>[1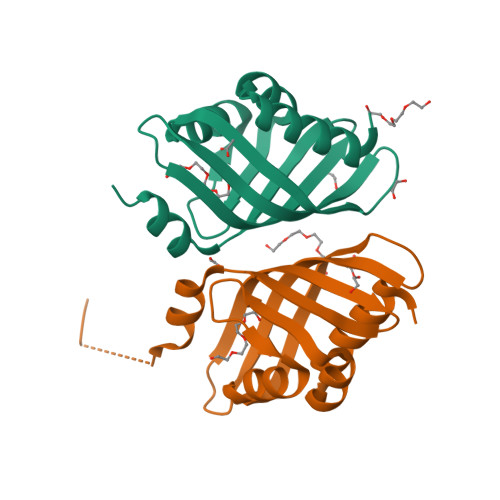6x]MTPLETVQLFLARVNALDLDGACALLAEDVVYDNVPMPTVHGRAAARAFLSQLPATAIDWETHAIAATGDAARGTVLTERTDRFTLADGRTLAIRVMGAFDVADGSITAWRDYFDLGQFMAQMAPSPSAHHHHHH>GPHTIIEEDTESTKTQREQEIIRLTQQLITSITAKDFDSYSKLVDPKITAFEPEALGNQVEGLEFHK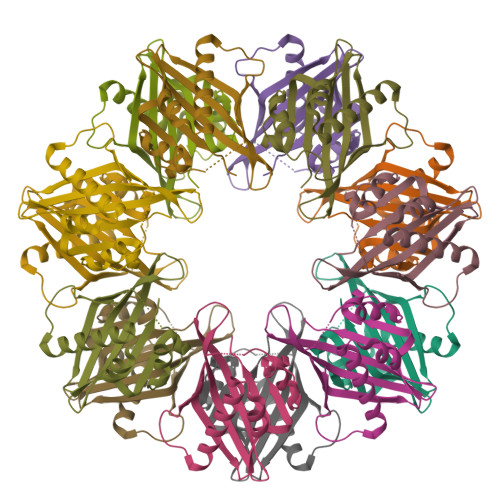FYFDNLPNKRNTTVNTTILAPHVQMLGEEGACISYVRLTQGIGPDGLPRTTQSEETRVWQKKKGVWLNVHFHRSVSRP[7x]>[2x]KETAAAKFERQHMDSSTSAASSSNYCNLMMCCRNLTKDRCKPVNTFVHESLADVQAVCSQKNVACKNGQTNCYQSYST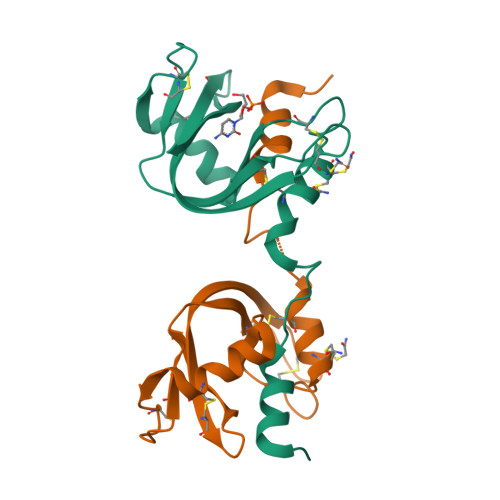MSITDCRETGSSKYPNCAYKTTQANKHIIVACEGNPYVPVHFDASV>AVPAPNQQPEVFCNQIFINNEWHDAVSRKTFPTVNPSTGEVICQVAEGDKEDVDKAVKAARAAFQLGSPWRRMDASHRGRLLNRLADLIERDRTYLAALETLDNGKPYVISYLVDLDMVLKCLRYYAGWADKYHGKTIPIDGDFFSYTRHEPVGVCGQIIPWNFPLLMQAWKLGPALATGNVVVMKVAEQTPLTALYVANLIKEAGFPPGVVNIVPGFGPTAGAAIASHEDVDKVAFTGSTEIGRVIQVAAGSSNLKRVTLELGGKSPNIIMSDADMDWAVEQAHFALFFNQGQCCCAGSRTFVQEDIYDEFVERS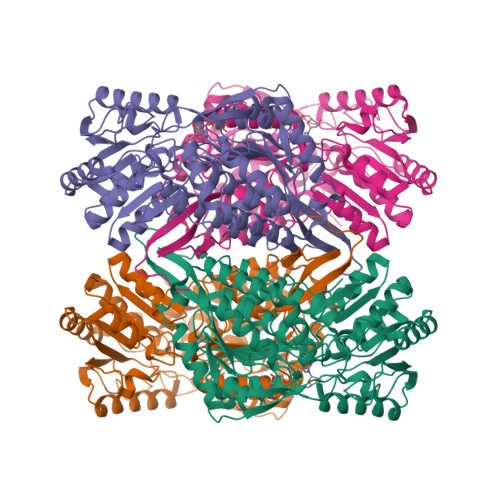VARAKSRVVGNPFDSKTEQGPQVDETQFKKILGYINTGKQEGAKLLCGGGIAADRGYFIQPTVFGDVQDGMTIAKEEIFGPVMQILKFKTIEEVVGRANNSTYGLAAAVFTKDLDKANYLSQALQAGTVWVNCYDVFGAQSPFGGYKMSGSGRELGEYGLQAYTEVKTVTVKVPQKNS[8x]The ecto-nucleotide pyrophosphatases/phosphodiesterases (ENPPs or NPPs) family consists of seven structurally-related ecto-enzymes. ENPP6 hydrolyzes only choline-containing lysophospholipids, such as LPC, sphingosylphosphorylcholine (SPC), platelet-activating factor (PAF) and lysoPAF, but not other lysophospholipids, suggesting that ENPP6 recognizes the choline moiety of its substrates. Here, we showed that GPC is hydrolyzed to phosphocholine by ENPP6, which is present on the extracellular surface of certain cells such as oligodendrocytes and liver sinusoid endothelial cells. In addition, we showed that ENPP6-deficient mice have impaired myelin structure and are prone to having a fatty liver, which are typical symptoms of choline deficiency. Together, these results strongly suggest that ENPP6 serves as a choline-supplying enzyme.

The extracellular PDE domain of mouse ENPP6 (residues 24–415) exists as a mixture of a monomer, dimer and higher-order oligomer, whereas the C393A/C412S mutant predominantly exists as a monomer25. The C393A/C412S mutant showed α-GPC-hydrolyzing activity comparable to the activities of the monomer and dimer of wild-type ENPP6, indicating that neither the oligomeric state nor the C393A/C412S mutation affects the enzymatic activity. We thus determined the crystal structures of the C393A/C412S mutant in the apo form (without substrates) at 2.0 Å resolution. Since the two structures are virtually identical (root-mean-square deviation [rmsd] of 0.23 Å for aligned Cα atoms), we will hereafter describe the ENPP6–phosphocholine complex structure, unless otherwise stated. Although electron densities of four glycans linked to Asn100, Asn118, Asn341 and Asn404 are observed in the apo form, the electron density of the Asn100-linked glycan was not observed in the complex, probably due to the flexibility of the Asn100-linked glycan. As observed in the structures of ENPP1, ENPP2 and ENPP4, two zinc ions are coordinated by conserved active-site residues. One zinc ion is coordinated by Asp193, His197 and His354, while the other is coordinated by Asp32, His241 and the catalytic nucleophile Ser71.

>MAAKLWTFLLGFGLSWVWPASAHRKLLVLLLDGFRSDYISEDALASLPGFREIVNRGVKVDYLTPDFPSLSYPNYYTLMTGRHCEVHQMIGNYMWDPRTNKSFDIGVNRDSLMPLWWNGSEPLWITLMKARRKVYMYYWPGCEVEILGVRPTYCLEYKTVPTDINFANAVSDALDSLKSGRADLAAIYHERIDVEGHHYGPSSPQRKDALRAVDTVLKYMIQWIQDRGLQQDLNVILFSDHGMTDIFWMDKVIELSNYISLDDLQQVKDRGPVVSLWPVPGKHSEIYHKLRTVEHMTVYEKESIPNRFYYKKGKFVSPLTLVADEGWFIAESREMLPFWMNSTGKREGWQRGWHGYDNELMDMRGIFLAIGPDFKSNFRAAPIRSVDVYNIMAHVAGITPLPNNGSWSRVVSMLKGQTSSASRENLYFQ[4x]>[12x]MRGSHHHHHHGSMNEIMICAVGNVATTPVFRDLANGPSVRFRLAVTARYWDREKNAWTDGHTNFFTVWANRQLATNASGSLAVGDPVVVQGRLKV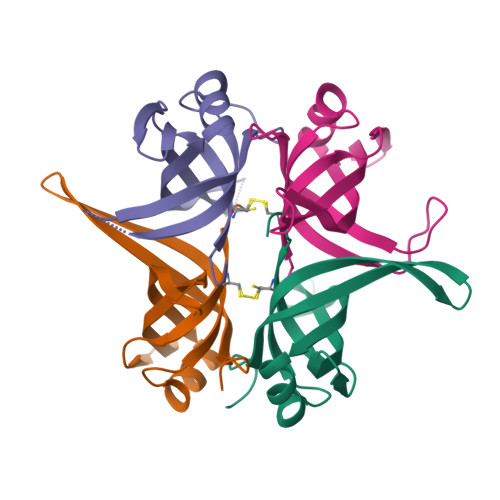RTDVREGQSRTSADIDAVAIGHDLARGTAAFRR> MTDTDDGGTMLPLPDFTATFPEPFPAGPHSERTEHRLLDWLEEHPLLPSAKAKAVLVNITSHGASRTFPTADADDLLLFAELLLWLTAFDDVHAEGNGVGGPAALVDRASELMLVLAGGNPPRAMSPFPAVLHDLLARFRARASAAAYHRLAASLRDTLMALVWEAHHVAKPEGVALATYLAMRPHTVFIKTITAAGEILLGYELTDTQRALAAVRNLETAVANLAGWINDLASYEREMQRGRGQPLSLPTLLHARHGGTIEEAFTRASSMCENEAAVARRGITHLAHASPNALTAHARALEDITRSFIWHTSHARYQGIRPNRGSSTSSPARSLQHHHH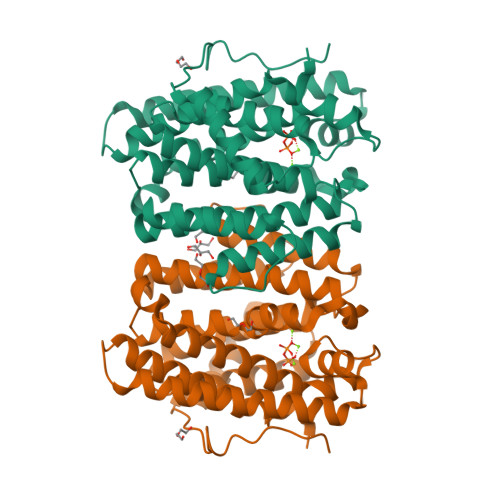HH> GDFAKEYADALYDSLGHSVLICDRDVYIAVSGSSKKDYLNKSISEMLERTMDQRSSVLESDAKSVQLVNGIDEDMNSYTVGPIVANGDPIGAVVIFSKDQTMG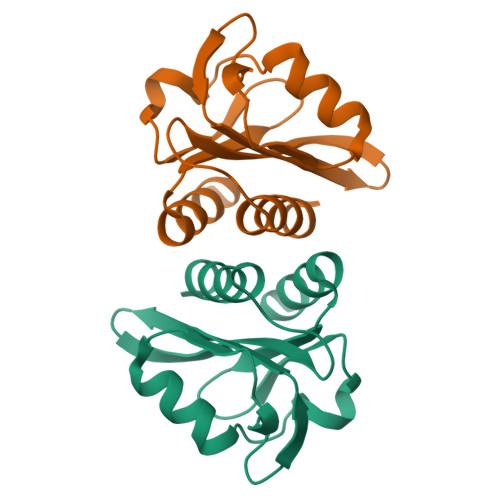EVEHKAVETAAGFLARQMEQ> GSVQALFDFDPQE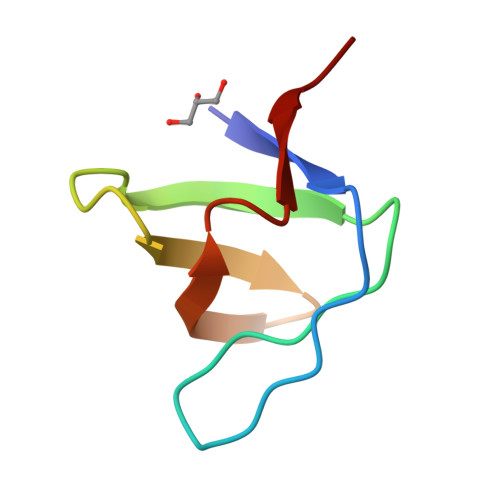DGELGFRRGDFIHVMDNSDPNWWKGACHGQTGMFPRNYVTPVN>[2x]MALQNEKNSRYLLRD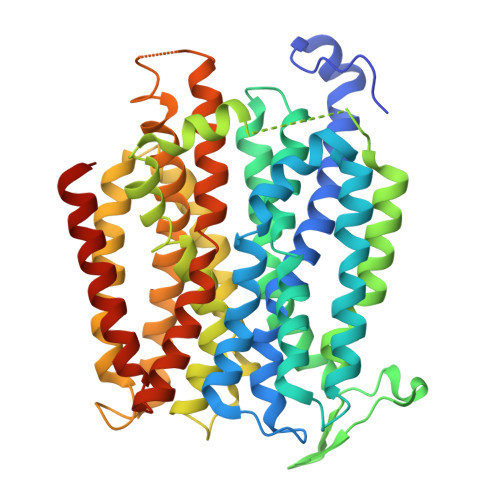WKPENPAFWENKGKHIARRNLWISVSCLLLAFCVWMLFSAVTVNLNKIGFNFTTDQLFLLTALPSVSGALLRVPYSFMVPIFGGRRWTVFSTAILIIPCVWLGIAVQNPNTPFGIFIVIALLCGFAGANFASSMGNISFFFPKAKQGSALGINGGLGNLGVSVMQLVAPLVIFVPVFAFLGVNGVPQADGSVMSLANAAWIWVPLLAIATIAAWSGMNDIASSRASIADQLPVLQRLHLWLLSLLYLATFGSFIGFSAGFAMLAKTQFPDVNILRLAFFGPFIGAIARSVGGAISDKFGGVRVTLINFIFMAIFSALLFLTLPGTGSGNFIAFYAVFMGLFLTAGLGSGSTFQMIAVIFRQITIYRVKMKGGSDEQAHKEAVTETAAALGFISAIGAVGGFFIPQAFGMSLNMTGSPVGAMKVFLIFYIVCVLLTWLVYGRRKFSQKLEVLFQ>MSSLSRELVFLILQFLDEEKFKETVHKLEQESGFFFNMKYFEEKVHAGEWDEVEKYLSGFTKVDDNRYSMKIFFEIRKQKYLEALDRHDRAKAVDILVKDLKVFSTFNEELYKEITQLLTLENFRENEQLSKYGDTKSAR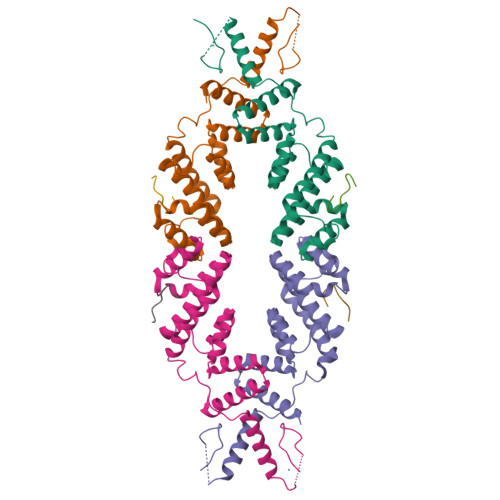SIMLIELKKLIEANPLFREKLVFPTLKASRLRTLINQSLNWQHQLCKNPRPNPDIKTLFTDHTCTPPNG[4x];>[4x]KDTELRLGLPG>[2x]MGHHHHHHSHMAFVTRQFMRSVSSSSTASASAKKIIVKHVTVIGGGLMGAGIAQVAAATGHTVVLVDQTEDILAKSKKGIEESLRKVAKKKFAENPKAGDEFVEKTLSTIATSTDAASVVHSTDLVVEAIVENLKVKNELFKRLDKFAAEHTIFASNTS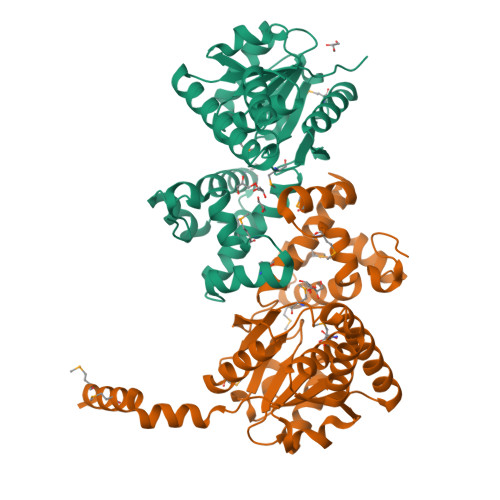SLQITSIANATTRQDRFAGLHFFNPVPVMKLVEVIKTPMTSQKTFESLVDFSKALGKHPVSCKDTPGFIVNRLLVPYLMEAIRLYERGDASKEDIDTAMKLGAGYPMGPFELLDYVGLDTTKFIVDGWHEMDAENPLHQPSPSLNKLVAENKFGKKTGEGFYKYK> MPVFHTRTIESILEPVAQQISHLVIMHEEGEVDGKAIPDLTAPVAAVQAAVSNLVRVGKETVQTTEDQILKRDMPPAFIKVENACTKLVQAAQMLQSDPYSVPARDYLIDGSRGILSGTSDLLLTFDEAEVRKIIRVCKGILEYLTVAEVVETMEDLVTYTKNLGPGMTKMAKMIDERQQELTHQEHRVMLVNSMNTVKELLPVLISAMKIFVTTKNSKNQGIEEALKNRNFTVEKMSAEINEIIRVLQLTSWDEDAWASKDTEAMKRALASIDSKLNQAKGWLRDPSASPGDAGEQAIRQILDEAGKVGELCAGKERREILGTCKMLGQMTDQVADLRARGQGSSPVAMQKAQQVSQGLDVLTAKVENAARKLEAMTNSKQSIAKKIDAAQNWLADPNGGPEGEEQIRGALAEARKIAELCDDPKERDDILRSLGEISALTSKLADLRRQGKGDSPEARALAKQVATALQNLQTKTNRAVANSRPAKAAVHLEGKIEQAQRWIDNPTVDDRGVGQAAIRGLVAEGHRLANVMMGPYRQDLLAKCDRVDQLTAQLADLAARGEGESPQARALASQLQDSLKDLKARMQEAMTQEVSDVFSDTTTPIKLLAVAATAPPDAPNREEVFDERAANFENHSGKLGATAEKAAAVGTANKSTVEGIQASVKTARELTPQVVSAARILLRNPGNQAAYEHFETMKNQWIDNVEKMTGLVDEAIDTKSLLDASEEAIKKDLDKCKVAMANIQPQMLVAGATSIARRANRILLVAKREVENSEDPKFREAVKAASDELSKTISPMVMDAKAVAGNISDPGLQKSFLDSGYRILGAVAKVREAFQPQEPDFPPPPPDLEQLRLTDELAPPKPPLPEGEVPPPRPPPPEEKDEEFPEQKAGEVINQPMMMAARQLHDEARKWSSKGNDIIAAAKRMA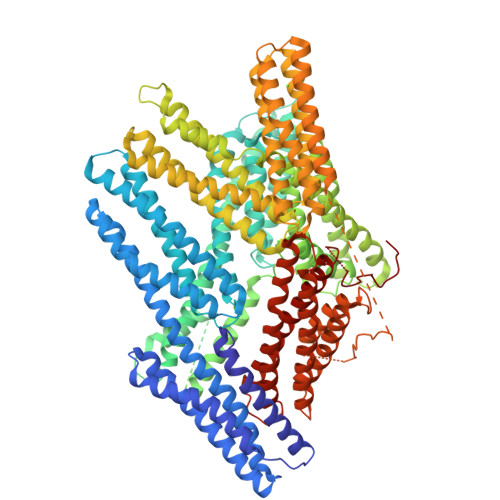LLMAEMSRLVRGGSGTKRALIQCAKDIAKASDEVTRLAKEVAKQCTKAAIATNLLQVCERIPTISTQLKILSTVKATMLGRTNISDEESEQATEMLVHNAQNLMQSVKETVREAEAASIKIRTDAGFTLRWVRKTPWYQ>AGPQLDVSCFAHDKNIGSRTEQLSVVHVASAQDCMKECQALPTCSHFTYNKNSKKCHLKAGAPEFYTYTGDMTGPRSCEHNCSDACWMDGNNPLAVWDYSGQPPALCWAACMGTPGCDLYTFQGMTCKLYSQTSSKRA[6x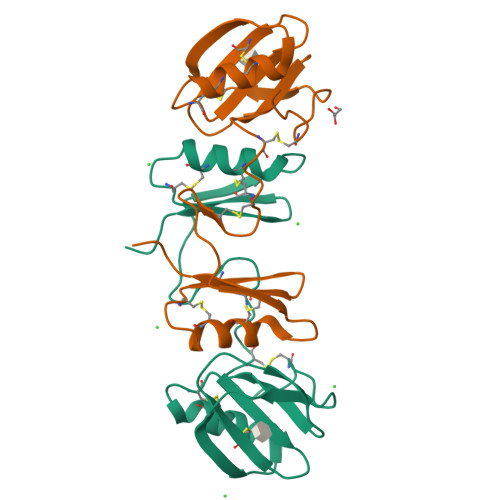]>[4x]GMSTQYWEEEIEIMSREKLQELQLQRLKKTINIAANSPYYKEVFSKNGITGDSIQSLDDIRKIPFTTKSDMRANYPFGLVAGDMK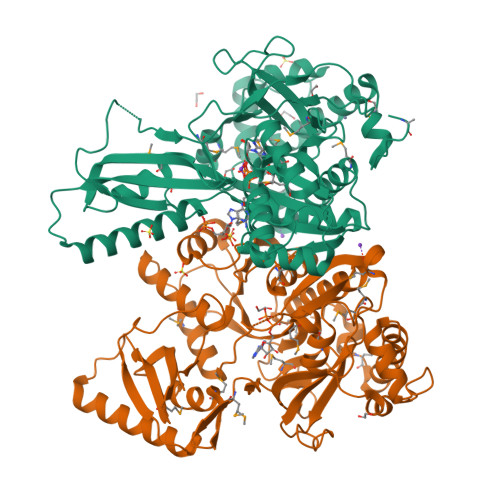RDGVRIHSSSGTTGNPTVIVHSQHDLDSWANLVARCLYMVGIRKTDVFQNSSGYGMFTGGLGFQYGAERLGCLTVPAAAGNSKRQIKFISDFKTTALHAIPSYAIRLAEVFQEEGIDPRETTLKTLVIGAEPHTDEQRRKIERMLNVKAYNSFGMTEMNGPGVAFECQEQNGMHFWEDCYLVEIIDPETGEPVPEGEIGELVLTTLDREMMPLIRYRTRDLTRILPGKCPCGRTHLRIDRIKGRSDDMFIIKGVNIFPMQVEKILVQFPELGSNYLITLETVNNQDEMIVEVELSDLSTDNYIELEKIRRDIIRQLKDEILVTPKVKLVKKGSLPQSEGKAVRVKDLRDNK> RLDAPSQIEVKDVTDTTALITWFKPLAEIDGIELTYGIKDVPGDRTTIDLT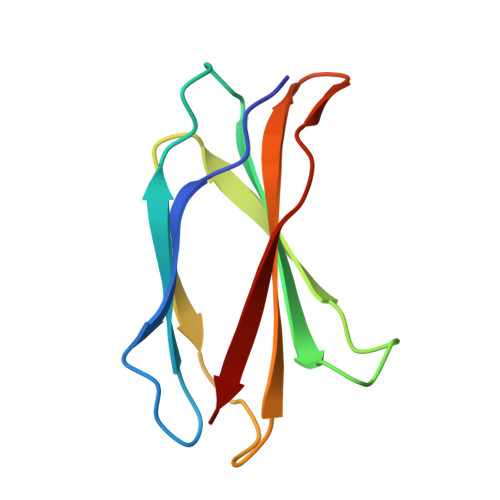EDENQYSIGNLKPDTEYEVSLISRRGDMSSNPAKETFTT3-methyl-L-alloisoleucine | 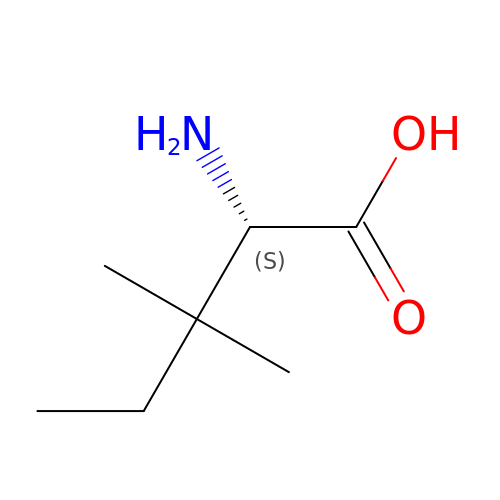C7 H15 N O2 | AQIFZAKDNFZWND-RXMQYKEDSA-N>[6x]GPHM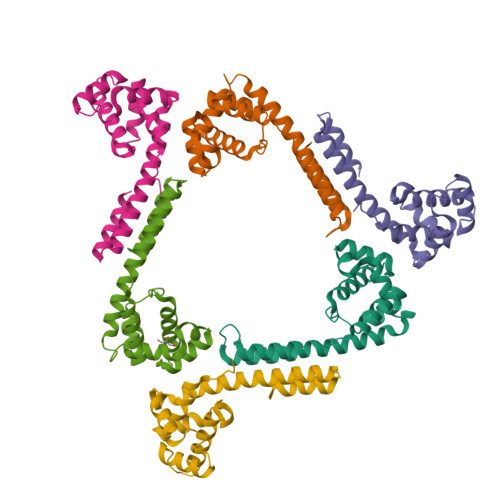AVVDDLAPGMDSSPPSEDYGRQPPQDLAAEQSVLGGMLLSKDAIADVLERLRPGDFYRPAHQNVYDAILDLYGRGEPADAVTVAAELDRRGLLRRIGGAPYLHTLISTVPTAANAGYYASIVAEKALLRRLVEAGTRVVQYGYAGAEGADVAEVVDRAQAEIYDVADRRLSEDFVALEDLLQPTMDEIDAIASSGG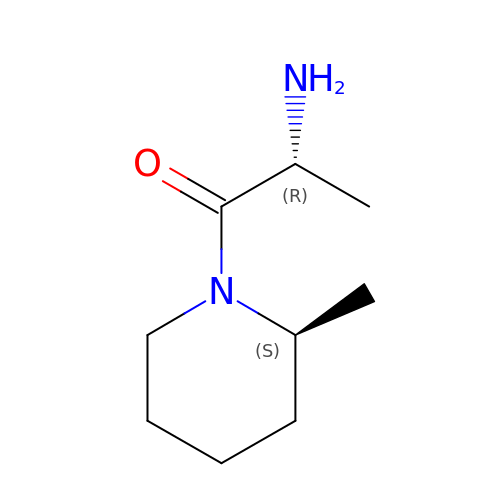(2R)-2-amino-1-[(2S)-2-methylpiperidin-1-yl]propan-1-one | C9 H18 N2 O | FZZIMRQDJKXDFD-JGVFFNPUSA-N> GATGRTTIAIDPVTRIEGHLKAEVVVENGKVVDARLSGGMYR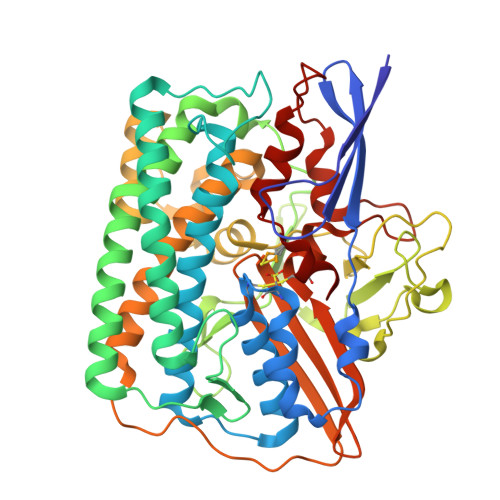GFETILRGRDPRDASQIVQRICGVCPTAHSTASVLALDEAFGAKVPNNGRITRNLIFGANYLQSHILHFYHLSAQDFVQGPDTAPFVPRFPKSDLRLSKELNKAGVDQYIEALEVRRICHEMVALFGGRMPHVQGQVVGGATEIPTKEKLVEYAARFKKVRDFVEQKYVPVVYTIGSKYKDMFKVGQGFKAALCVGAFPLDNSGKKHLFMPGVYAKGKDMPFDPSKIKEYVKYSWFAEETTGLNYKEGKTIPAPDKAGAYSFVKAPRYDGLSLEVGPLARMWVNNPELSPVGKKLLKDLFGISAKKFRDLGEEAAFSLMGRHVARAEETYYMLGAIEGWLKEIKAGEDTVVMPAVPASAEGTGFTEAPRGSLLHYVKVKDSKIDNYQIVSASLWNCNPRDDMGQRGAVEEALIGIPVDDIQNPVNVARLIRAFDPULGCAVH> WPHSIESSNDWNVEKRSIRDVPVVRLPADS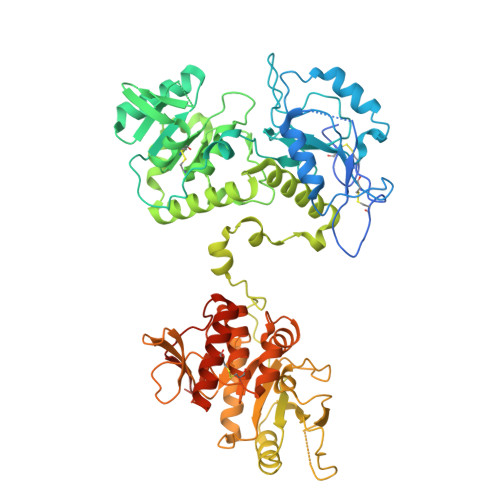PIPERGDLSCRMHTCFDVYRCGFNPKNKIKVYIYALKKYVDDFGVSVSNTISREYNELLMAISDSDYYTDDINRACLFVPSIDVLNQNTLRIKETAQAMAQLSRWDRGTNHLLFNMLPGGPPDYNTALDVPRDRALLAGGGFSTWTYRQGYDVSIPVYSPLSAEVDLPEKGPGPRQYFLLSSQVGLHPEYREDLEALQVKHGESVLVLDKCTNLSEGVLSVRKRCHKHQVFDYPQVLQEATFCVVLRGARLGQAVLSDVLQAGCVPVVIADSYILPFSEVLDWKRASVVVPEEKMSDVYSILQSIPQRQIEEMQRQARWFWEAYFQSIKAIALATLQIINDRIYPYAAISYEEWNDPPAVKWGSVSNPLFLPLIPPQSQGFTAIVLTYDRVESLFRVITEVSKVPSLSKLLVVWNNQNKNPPEDSLWPKIRVPLKVVRTAENKLSNRFFPYDEIETEAVLAIDDDIIMLTSDELQFGYEVWREFPDRLVGYPGRLHLWDHEMNKWKYESEWTNEVSMVLTGAAFYHKYFNYLYTYKMPGDIKNWVDAHMNCEDIAMNFLVANVTGKAVIKVTPRKKFKCPECTAIDGLSLDQTHMVERSECINKFASVFGTMPLKVVEHRADPVLYKDDFPEKLKSFPNIGSL>GSSSGGSGHTPTTQATHADDHDLTTHNGTEEHDDGHDDGHDDLHAHAPKVIVFISGSCLFGAISRSLFKKLPIPYTVVLLILGAILGVVASNVPLVEEHTRDVAHMDPHVLLQIFLPVLIFESAFAMDVHTFMRSFSQVCILALFGLVVASVLTAVLAMNLFNYNWNFSEAMMFGAIMSATDPVAVVALLKDLGASKQLGTIIEGESLLNDGCAIVIFNVFMKMVFFPQLTSTVGQNVLYFLQVAVAGPLWGYAVAKVTVFFLSHIFNDALVEITITLAATYLTYYIGDIWLEVSGVLAVVVLGLIVNAEKTSISPEVEVFLHRFWEMLAYLANTLIFMMVGVVVTQKALVAVDKMDWFYLIILYLAITIIRGMVISLFSPILSRIGYGLTWRNAVIMTWGGLRGAVGLALALVVENLAGNDVIGSKFLFHTAGIVVLTLVINATTIQTLLRILGMSDISIPKRLAMAGAVRRIHEGQNRTLNMLKSDRFLADADWDIATAACEISDPYSALSDDENAPADELTLGERKSVCPGCKAMVPNEPSPREFADMMEEARLRMLKAEKISYWKQFEHGMLAREALRLLVQHAEVAADEKDQFILVDDLKKSWQIKGIYPWLKRKLEDLISEKKIAAIPMPKYKLGKLMYKICHHMAFEVTINIAIVLNIVPIIMEFVVQDKMASVSTMAAPGSTVSSEPSSLQKIEDALRISNYVFFVIYAIEAIVKILGLGRHYIVSHWNKFDAFILVVALVDIIIAETLLKGSITINLSSIKVVKLFRLLRGLRMLRLTKALIPKLILVVNGKINNQLSLGYDVGKGYIIGEEEVGKIIDRMVDNKKILRELKHISETGRLQVVKELGLLQREHPGIAVSVKTRQAIRTILNHSRETIHELQGAGLLDEMEAHKLELTVEIKMKRLMNAPSSIPPPPPENLLKNVSWLAGDMKLIDFIKARASLLHFDYGEVIVREGDESDGLFLIVSG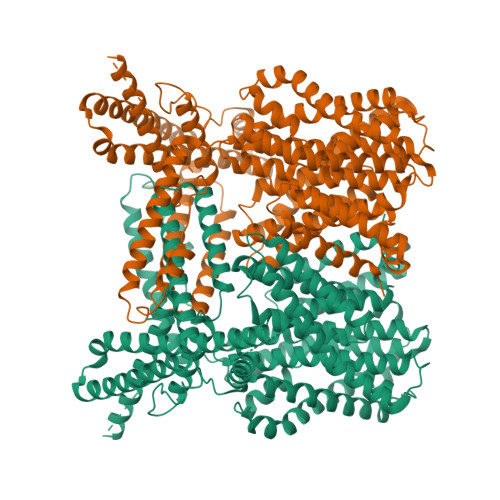LVKLYGKSAFLDHDNPPVTAGSEENEVFEDYLTVGNVIGEMGVLTKKPRNATVTCETTVQVYFITAEDMNIAIDTFTLYPSLEYRLWRVVAIRIATPLIMEQMAFQGWTQEKVKLHLERGYLVDLAESHFQFNIDATLEDVILINGTAYNAHTREEIRSPCLISRTVHKLTFQYTATEEPRLFVVRNAEYNGPILDGRLDVDSKRSLISITEISSNMCLKHAAELRQKNSKVMLSRKSSGAAAKEEEDCIPNTSDVEQAAGVSPSVPTKTTPKPKSFLPSLGLSMSKERVNGEAVEESPVKTKQGEETPETEEGAAPRVNVASNSLEVLFQ[2x]> GPMVTGGGAAPPGTVTEPLPSVIVLSAGRKMAAAAAAASGPGCSSAAGAGAAGVSEWLVLRDGCMHCDADGLHSLSYHPALNAILAVTSRGTIKVIDGTSGATLQASALSAKPGGQVKCQYISAVDKVIFVDDYAVGCRKDLNGILLLDTALQTPVSKQDDVVQLELPVTEAQQLLSACLEKVDISSTEGYDLFITQLKDGLKNTSHETAANHKVAKWATVTFHLPHHVLKSIASAIVNELKKINQNVAALPVASSVMDRLSYLLPSARPELGVGPGRSVDRSLMYSEANRRETFTSWPHVGYRWAQPDPMAQAGFYHQPASSGDDRAMCFTCSVCLVCWEPTDEPWSEHERHSPNCPFVKGEHTQNVPLSVTLATSPAQFPCTDGTDRISCFGSGSCPHFLAAATKRGKICIWDVSKLMKVHLKFEINAYDPAIVQQLILSGDPSSGVDSRRPTLAWLEDSSSCSDIPKLEGDSDDLLEDSDSEEHSRSDSVTGHTSQKEAMEVSLDITALSILQQPEKLQWEIVANVLEDTVKDLEELGANPCLTNSKSEKTKEKHQEQHNIPFPCLLAGGLLTYKSPATSPISSNSHRSLDGLSRTQGESISEQGSTDNESCTNSELNSPLVRRTLPVLLLYSIKESDEKAGKIFSQMNNIMSKSLHDDGFTVPQIIEMELDSQEQLLLQDPPVTYIQQFADAAANLTSPDSEKWNSVFPKPGTLVQCLRLPKFAEEENLCIDSITPCADGIHLLVGLRTCPVESLSAINQVEALNNLNKLNSALCNRRKGELESNLAVVNGANISVIQHESPADVQTPLIIQPEQRNVSGGYLVLYKMNYATRIVTLEEEPIKIQHIKDPQDTITSLILLPPDILDNREDDCEEPIEDMQLTSKNGFEREKTSDISTLGHLVITTQGGYVKILDLSNFEILAKVEPPKKEGTEEQDTFVSVIYCSGTDRLCACTKGGELHFLQIGGTCDDIDEADILVDGSLSKGIEPSSEGSKPLSNPSSPGISGVDLLVDQPFTLEILTSLVELTRFETLTPRFSATVPPCWVEVQQEQQQRRHPQHLHQQHHGDAAQHTRTWKLQTDSNSWDEHVFELVLPKACMVGHVDFKFVLNSNITNIPQIQVTLLKNKAPGLGKVNALNIEVEQNGKPSLVDLNEEMQHMDVEESQCLRLCPFLEDHKEDILCGPVWLASGLDLSGHAGMLTLTSPKLVKGMAGGKYRSFLIHVKAVNERGTEEICNGGMRPVVRLPSLKHQSNKGYSLASLLAKVAAGKEKSSNVKNENTSGTRKSENLRGCDLLQEVSVTIRRFKKTSISKERVQRCAMLQFSEFHEKLLNTLCRKTDDGQITEHAQSLVLDTLCWLAGVHSNGPGSSKEGNENLLSKTRKFLSDIVRVCFFEAGRSIAHKCARFLALCISNGKCDPCQPAFGPVLLKALLDNMSFLPAATTGGSVYWYFVLLNYVKDEDLAGCSTACASLLTAVSRQLQDRLTPMEALLQTRYGLYSSPFDPVLFDLEMSGSSCKNVYNSSIGVQSDEIDLSDVLSGNGKVSSCTAAEGSFTSLTGLLEVEPLHFTCVSTSDGTRIERDDAMSSFGVTPAVGGLSSGTVGEASTALSSAAQVALQSLSHAMASAEQQLQVLQEKQQQLLKLQQQKAKLEAKLHQTTAAAAAAASAVGPVHNSVPSNPVAAPGFFIHPSDVIPPTPKTTPLFMTPPLTPPNEAVSVVINAELAQLFPGSVIDPPAVNLAAHNKNSNKSRMNPLGSGLALAISHASHFLQPPPHQSIIIERMHSGARRFVTLDFGRPILLTDVLIPTCGDLASLSIDIWTLGEEVDGRRLVVATDISTHSLILHDLIPPPVCRFMKITVIGRYGSTNARAKIPLGFYYGHTYILPWESELKLMHDPLKGEGESANQPEIDQHLAMMVALQEDIQCRYNLACHRLETLLQSIDLPPLNSANNAQYFLRKPDKAVEEDSRVFSAYQDCIQLQLQLNLAHNAVQRLKVALGASRKMLSETSNPEDLIQTSSTEQLRTIIRYLLDTLLSLLHASNGHSVPAVLQSTFHAQACEELFKHLCISGTPKIRLHTGLLLVQLCGGERWWGQFLSNVLQELYNSEQLLIFPQDRVFMLLSCIGQRSLSNSGVLESLLNLLDNLLSPLQPQLPMHRRTEGVLDIPMISWVVMLVSRLLDYVATVEDEAAAAKKPLNGNQWSFINNNLHTQSLNRSSKGSSSLDRLYSRKIRKQLVHHKQQLNLLKAKQKALVEQMEKEKIQSNKGSSYKLLVEQAKLKQATSKHFKDLIRLRRTAEWSRSNLDTEVTTAKESPEIEPLPFTLAHERCISVVQKLVLFLLSMDFTCHADLLLFVCKVLARIANATRPTIHLCEIVNEPQLERLLLLLVGTDFNRGDISWGGAWAQYSLTCMLQDILAGELLAPVAAEAMEEGTVGDDVGATAGDSDDSLQQSSVQLLETIDEPLTHDITGAPPLSSLEKDKEIDLELLQDLMEVDIDPLDIDLEKDPLAAKVFKPISSTWYDYWGADYGTYNYNPYIGGLGIPVAKPPANTEKNGSQTVSVSVSQALDARLEVGLEQQAELMLKMMSTLEADSILQALTNTSPTLSQSPTGTDDSLLGGLQAANQTSQLIIQLSSVPMLNVCFNKLFSMLQVHHVQLESLLQLWLTLSLNSSSTGNKENGADIFLYNANRIPVISLNQASITSFLTVLAWYPNTLLRTWCLVLHSLTLMTNMQLNSGSSSAIGTQESTAHLLVSDPNLIHVLVKFLSGTSPHGTNQHSPQVGPTATQAMQEFLTRLQVHLSSTCPQIFSEFLLKLIHILSTERGAFQTGQGPLDAQVKLLEFTLEQNFEVVSVSTISAVIESVTFLVHHYITCSDKVMSRSGSDSSVGARACFGGLFANLIRPGDAKAVCGEMTRDQLMFDLLKLVNILVQLPLSGNREYSARVSVTTNTTDSVSDEEKVSGGKDGNGSSTSVQGSPAYVADLVLANQQIMSQILSALGLCNSSAMAMIIGASGLHLTKHENFHGGLDAISVGDGLFTILTTLSKKASTVHMMLQPILTYMACGYMGRQGSLATCQLSEPLLWFILRVLDTSDALKAFHDMGGVQLICNNMVTSTRAIVNTARSMVSTIMKFLDSGPNKAVDSTLKTRILASEPDNAEGIHNFAPLGTITSSSPTAQPAEVLLQATPPHRRARSAAWSYIFLPEEAWCDLTIHLPAAVLLKEIHIQPHLASLATCPSSVSVEVSADGVNMLPLSTPVVTSGLTYIKIQLVKAEVASAVCLRLHRPRDASTLGLSQIKLLGLTAFGTTSSATVNNPFLPSEDQVSKTSIGWLRLLHHCLTHISDLEGMMASAAAPTANLLQTCAALLMSPYCGMHSPNIEVVLVKIGLQSTRIGLKLIDILLRNCAASGSDPTDLNSPLLFGRLNGLSSDSTIDILYQLGTTQDPGTKDRIQALLKWVSDSARVAAMKRSGRMNYMCPNSSTVEYGLLMPSPSHLHCVAAILWHSYELLVEYDLPALLDQELFELLFNWSMSLPCNMVLKKAVDSLLCSMCHVHPNYFSLLMGWMGITPPPVQCHHRLSMTDDSKKQDLSSSLTDDSKNAQAPLALTESHLATLASSSQSPEAIKQLLDSGLPSLLVRSLASFCFSHISSSESIAQSIDISQDKLRRHHVPQQCNKMPITADLVAPILRFLTEVGNSHIMKDW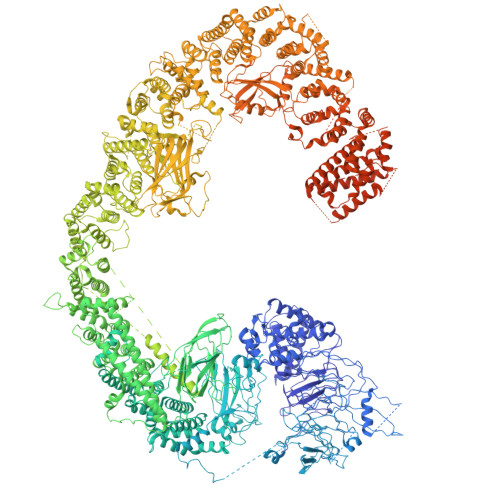LGGSEVNPLWTALLFLLCHSGSTSGSHNLGAQQTSARSASLSSAATTGLTTQQRTAIENATVAFFLQCISCHPNNQKLMAQVLCELFQTSPQRGNLPTSGNISGFIRRLFLQLMLEDEKVTMFLQSPCPLYKGRINATSHVIQHPMYGAGHKFRTLHLPVSTTLSDVLDRVSDTPSITAKLISEQKDDKEKKNHEEKEKVKAENGFQDNYSVVVASGLKSQSKRAVSATPPRPPSRRGRTIPDKIGSTSGAEAANKIITVPVFHLFHKLLAGQPLPAEMTLAQLLTLLYDRKLPQGYRSIDLTVKLGSRVITDPSLSKTDSYKRLHPEKDHGDLLASCPEDEALTPGDECMDGILDESLLETCPIQSPLQVFAGMGGLALIAERLPMLYPEVIQQVSAPVVTSTTQEKPKDSDQFEWVTIEQSGELVYEAPETVAAEPPPIKSAVQTMSPIPAHSLAAFGLFLRLPGYAEVLLKERKHAQCLLRLVLGVTDDGEGSHILQSPSANVLPTLPFHVLRSLFSTTPLTTDDGVLLRRMALEIGALHLILVCLSALSHHSPRVPNSSVNQTEPQVSSSHNPTSTEEQQLYWAKGTGFGTGSTASGWDVEQALTKQRLEEEHVTCLLQVLASYINPVSSAVNGEAQSSHETRGQNSNALPSVLLELLSQSCLIPAMSSYLRNDSVLDMARHVPLYRALLELLRAIASCAAMVPLLLPLSTENGEEEEEQSECQTSVGTLLAKMKTCVDTYTNRLRSKRENVKTGVKPDASDQEPEGLTLLVPDIQKTAEIVYAATTSLRQANQEKKLGEYSKKAAMKPKPLSVLKSLEEKYVAVMKKLQFDTFEMVSEDEDGKLGFKVNYHYMSQVKNANDANSAARARRLAQEAVTLSTSLPLSSSSSVFVRCDEERLDIMKVLITGPADTPYANGCFEFDVYFPQDYPSSPPLVNLETTGGHSVRFNPNLYNDGKVCLSILNTWHGRPEEKWNPQTSSFLQVLVSVQSLILVAEPYFNEPGYERSRGTPSGTQSSREYDGNIRQATVKWAMLEQIRNPSPCFKEVIHKHFYLKRVEIMAQCEEWIADIQQYSSDKRVGRTMSHHAAALKRHTAQLREELLKLPCPEGLDPDTDDAPEVCRATTGAEETLMHDQVKPSSSKELPSDFQL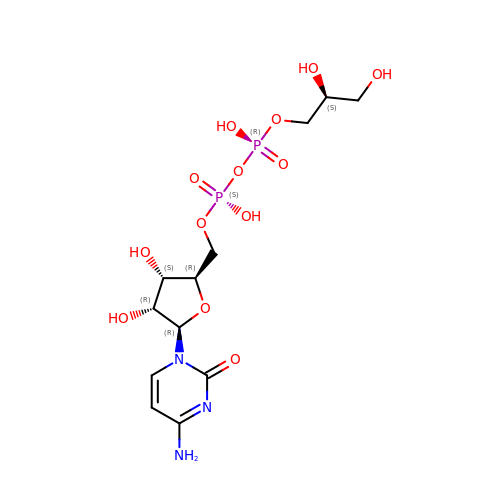[CYTIDINE-5'-PHOSPHATE] GLYCERYLPHOSPHORIC ACID ESTER | C12 H21 N3 O13 P2 | HHPOUCCVONEPRK-CNYIRLTGSA-N> XGGTLAIQAQGDLTLAQKKIVRKTWHQLMRNKTSFVT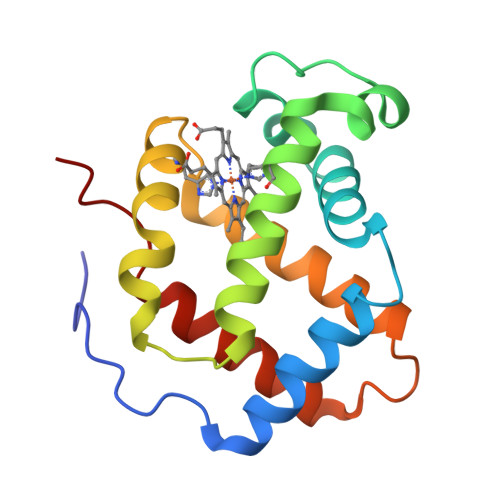DVFIRIFAYDPSAQNKFPQMAGMSASQLRSSRQMQAHAIRVSSIMSEYVEELDSDILPELLATLARTHDLNKVGADHYNLFAKVLMEALQAELGSDFNEKTRDAWAKAFSVVQAVLLVKHG> VDEMDTHDPHQLRYEKFFFTVKMTVRSNRPFRTYSDVAAAVSHWDHMYIGMAGKRPFYKILAFLGSSNLKATPAVLADQGQPEYHAHCEGRAYLPHRMGKTPPMLNVPEHFRRPF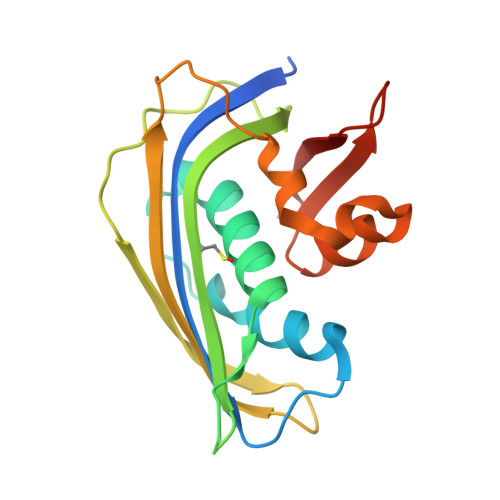NIGLYKGTVELTMTIYDDESLEAAPMIWDHFNSSKFSDFREKALMFGLIVEKKASGAWVLDSVSHFK In contrast to its eukaryotic counterparts, bacterial HSS synthesizes 1 mol HSP from 2 mol PUT. NAD+ serves as a non-covalently bound prosthetic group for BvHSS. The interface area of the dimer was calculated as approximately 1700 Å2 by PDBsum indicating a stable dimer23. The BvHSS subunit consists of two domains as determined by CATH24: one “NAD(P)-binding Rossmann-like” domain (domain 1, residues 3–163 and 394–425) and one “homospermidine-synthase-like domain” (domain 2, residues 164–395 and 426–477) as shown in Fig. 2a and S1. The crystal structures of BvHSS containing NAD+ clearly show that the active site is localized inside each subunit.

The phosphate-binding motif (18GFGSIG23) is located in the loop connecting β-strand 2 and α-helix A of the Rossmann fold. The adenosine part of NAD+ is bound via loop regions located between β-strand 4, 5, 6 and α-helix C, D, E. Nicotineamide-riboside-binding residues are found in loop regions between β-strand 7 and 8 and α-helix F and O. The pocket is a “boot-shaped” cavity that is approximately 21 Å deep. The entry to the pocket is formed by part of the “track-and-trace” loop (residues Phe-122 to Asp-125) and the α-helix J at the protein surface. The innermost end lies near amino acids Asn-162 and Glu-210. The active site is situated between residues Asn-162, Trp-229, Glu-237, His-296, and the nicotine amide ring of NAD+ at the narrow end of the pocket. Residues Val-115, Val-116, Tyr-123, Asn-135, Leu-138, Pro-163, Gln-240, Thr-295, and Asn-297 form a side pocket at the “heel” of the “boot-shaped” binding pocket, which is filled with six ordered water molecules of which five occur in a nearly planar and equidistant five-membered ring. At least five amino acids (Val-93, Glu-117, Tyr-123, Gly-233, and Ser-236) form a pore at the binding pocket entrance.

>GPMTDWPVYHRIDGPIVMIGFGSIGRGTLPLIERHFAFDRSKLVVIDPSDEARKLAEARGVRFIQQAVTRDNYRELLVPLLTAGPGQGFCVNLSVDTSSLDIMELARENGALYIDTVVEPWLGFYFDPDLKPEARSNYALRETVLAARRNKPGGTTAVSCCGANPGMVSWFVKQALVNLAADLGVTGEEPTTREEWARLAMDLGVKGIHIAERDTQRASFPKPFDVFVNTWSVEGFVSEGLQPAELGWGTFERWMPDNARGHDSGCGAGIYLLQPGANTRVRSWTPTAMAQYGFLVTHNESISIADFLTVRDAAGQAVYRPTCHYAYHPCNDAVLSLHEMFGSGKRQSDWRILDETEIVDGIDELGVLLYGHGKNAYWYGSQLSIEETRRIAPDQNATGLQVSSAVLAGMVWALENPNAGIVEADDLDFRRCLEVQTPYLGPVVGVYTDWTPLAGRPGLFPEDIDTSDPWQFRNVLVRD[2x]>[2x]MTATVGRWMGPAEYQQMLDTGTVVQSSTGTTHVAYPADIDAFGKQAKNGAMYVEFDVPEKSLVPT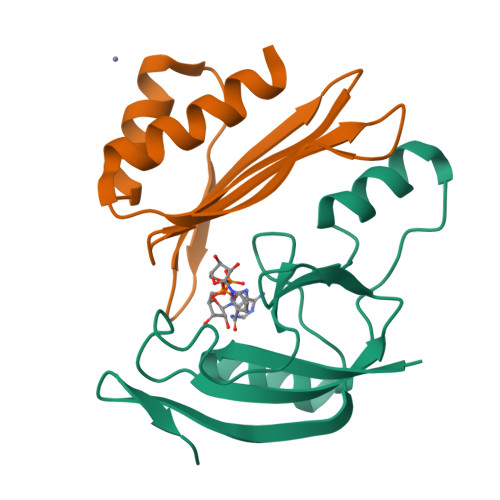NEGWAKIVGPDSIEGRLAKRKGLPVPEMPTAENITVRGEKINGEVEAKC;>MLNKFKLWVSKHTDYTVIHNENDLSYSIIIDFEDDRYISRFTVWDDLSCMSEVMDVDTGLYKLNKRNEFSTFDELLDIFDDFMISIK[2x]>TAELKICRVNRRSGSCLGGDEIFLLCDKVQKEDIEVYFTGPGWEARGSFSQADVHRQVAIVFRTPPYADPSLQAPVRVSMQLRRPSDRELSEPMEFQYLPDTDDRHR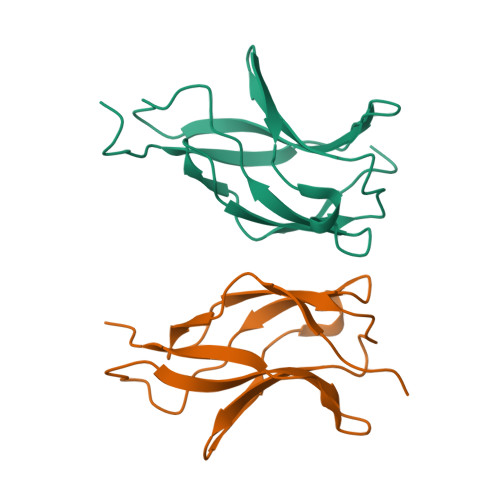IEEKRKR[2x]>MTKQHAFTREDLLRCSRGELFGPGNAQLPAPNMLMIDRIVHISDVGGKYGK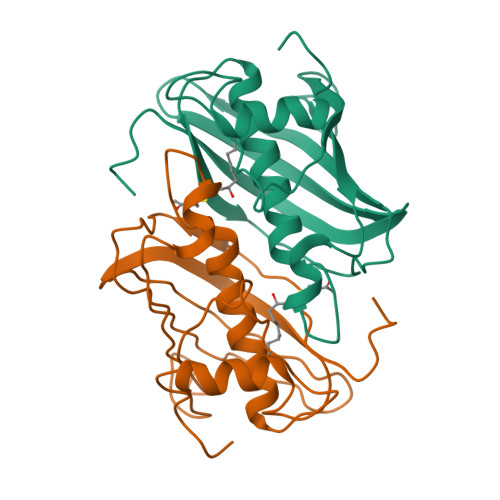GELVAELDINPDLWFFACNFEGDPVMPGCLGLDAMWQLVGFYLGWQGNPGRGRALGSGEVKFFGQVLPTAKKVTYNIHIKRTINRSLVLAIADGTVSVDGREIYSAEGLRVGLFTSTDSF[5x]>HHHHHHTHVDTVKVINDPIHGHIELHPLLIRIIDTPQFQRLRYIKQLGGGYYVFPGASHNRFEHSLGVGYLAGCLVRELSEKQPELQISERDMLCVQIAGLCRNLG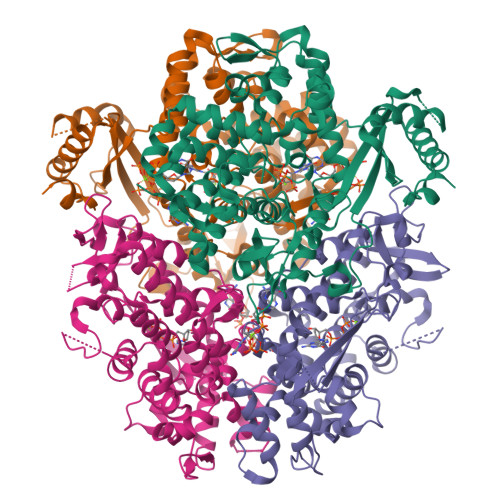HGPFSHMFDGRFIPLARPDVKWTHEQGSVNMFEHLVNSNGLIDVMEHYGLIPEEDIWFIKEQITGPLESPVKNATWPYKGRPKEKSFLYEIVANKRNGIDVDKWDYFARDCHHLGIQNNFDYKRFIKFARVCEVDNKKHICTREKEVGNLYDMFHTRNCLHRRAYQHKVGNIIDTMITDAFLKADPYIEITGSEGKKYRISTAIDDMEAFTKLTDNIFLEILYSTDPKLDAARAILKKIECRNLYKFVGETQPGRQDKIKRENYESLPKGVASAKPSNIQLEAELKAEDFIVDVINMDYGMEDKNPIDNVRFYCKSDPNKAIIITKNQVSQLLPERFAEQLIRVYCKKTDEKSLFAARQHFVQWCLDNDFTKPQDGDVVAPLITPRKLEWNSTHSAQSQARTREASKSRVRLFAKDSV[8x]>[2x]AMSRSRPELGDWSSPAELAELQRSQLPRVLAQALRSPFYAARYRGTTPPRTADDFAGVEVTAKQDLRDQYPFGMLAVGREHLATYHESSGTAGEPTASYYTEEDWTDLAERFARKWTGIHPSDTFLVRTPYGLVITGHLAQAAGRLRGATVVPGDARSLATPLSRMVRVLKTLDVTLTWCNPTEITMLAAAAKAAGLRPDQDFPHLRAMFTAAEPLTEVRRRRLSEIWGGIPVVEEYGSTETGTIAGQCPEGRMHLWADRAIFEVYDPRTGTLSEAGRGQMVVTPLYRDAMPLLRYNLADDVEVSTDPCGCGWLLPTVTVLGRAGTGHRIGPATVTQQRLEELVFSLPAAYEVMFWRAKAHPDVLELEFEAPEPVRQRAVKELGAALDRELGVPHRITGLAPGTLVPAEALTAQRDILKARYLFAEDEDWDKAVMYF

We reconstituted the biosynthesis of the benzoxazole moiety found in nataxazole by adding two enzymes (NatL2, NatAM), to 3‐HAA, ATP, and Mg2+. We have determined the structures of both NatL2 (homologue of BomJ) and NatAM (homologue of BomN) from the antitumor nataxazole pathway. We show NatL2 catalyzes ester not, as previously reported, amide formation; the amide is a shunt product. NatAM catalyzes benzoxazole from this ester by a mechanism that we propose involves shuttling of protons to control the fate of a hemiorthoamide intermediate.

We soaked the AMP crystals with both AMPPNP and 3‐HAA overnight and saw clear density for both molecules. The adenosine and ribose rings of AMPPNP in this complex overlap with their positions in the AMPPNP binary complex. The α‐ and β‐phosphates in the AMPPNP:3‐HAA ternary complex have however shifted and overlap with the β‐ and γ‐phosphates in the AMPPNP. In the AMPPNP:3‐HAA ternary complex, the γ‐phosphate salt bridges to Lys62 and Arg68. The 3‐HAA molecule binds in a pocket adjacent to the AMPPNP positioning one oxygen of the carboxylate group 3.3 Å from the α‐phosphate with an angle of attack of 167° (Ocarboxylate–Pα–Ophosphoanhydride) consistent with adenylation of the carboxylate. Thr239 hydrogen bonds to both α‐phosphate and carboxylate oxygen atoms. The hydroxyl group of 3‐HAA is hydrogen bonded to Glu235 whilst the amino group makes a hydrogen bond to N7 of the adenosine ring. The benzene ring stacks against a stretch of the main chain of Gly237 and Ser238. This complex is model for the Michealis complex of the first half (adenylation) reaction.In the present work, we focus on a class of monocyclic disulfide‐containing 19 amino acid peptides targeting the Vascular Endothelial Growth Factor‐A, the main pro‐angiogenic factor in Human. We proposed to use this peptide as a model to rationalize the thermodynamics of α‐helix stabilization by an i to i+4 lactam bridge. Around 950 Å2 of accessible surface area (ASA) was buried at the peptide‐VEGF interface, that overlapped with the VEGF receptor 1 domain 2 (VEGFR1‐d2)‐binding site. Although only lactam‐bridged ExxxK, DxxxK and KxxxD induced the formation of stable helix in the unbound state, all peptides of the series were helically folded when bound to VEGF.

Constraints caused by the lactam bridges and by the binding of the macro‐cyclized peptide to the VEGF site also made the α‐helices non‐canonical: in each of the four peptides, the residues P8‐11 folded into a 310‐helix characterized by a H‐bond between Glu P8 O and Cys P11 HN. In the peptide 3 c (ExxxK) the α‐helix extended from residues P9 to P12 followed by a 310 turn where Phe P12 O was H‐bound to Leu P15 HN. Interestingly the lactam bridge cyclization caused the side chains of residues P10 and P14 for peptide 1 c and 3 c to be in a non standard rotamer conformation, the consequence of which was moderate steric clashes involving hydrogen atoms. Therefore, lactam cyclization can result in sub‐optimal geometry with remaining steric constraints, where the side chains did not adopt the standard conformers (1 c and 3 c peptides). The real space correlation coefficient (RSCC) of the α‐helix was higher than 0.83 on VEGF:1 c, VEGF:2 c and VEGF:3 c structures, which supported these models. However, the NMR structure calculations did not converge into a single conformation. The backbone RMSD of the 20 lowest energy NMR structures, compared to the co‐crystal structures of bicyclic peptides and VEGF (see below), indicated that the bicyclic 2 c and 3 c were significantly closer to the folded structures than were the other peptides. In particular, the RMSD values in the α‐helix segment P10‐14 were extremely low for these bicyclic peptides (1.1 and 0.6 Å), showing their similarity with the crystal structure (see the supplementary NMR discussion for a more detailed description, including the β‐turn P2‐5 and extended fragment P6‐9). Helical folds were observed in most structures for 2 c and 3 c, resulting in a single α‐helical cluster for a RMSD cutoff of 1.2 Å. The location at lower ΔH and ‐TΔS of the preorganized peptides 1 c, 2 c and 3 c at 20 °C and 37 °C directly reflected the lower ΔG values in comparison to the other unfolded peptides.

> CDIHVLWEWECFEKL;>EVVKFMDVYQRSYCHPIETLVDIFQEYPDEIEYIFKPSCVPLMRCGGCCNDEGLECVPTEESNITMQIMRIKPHQGQHIGEMSFLQHNKCECRPK[2x]>[2x]WELTILHTNDVHSRLEQTSEDSSKC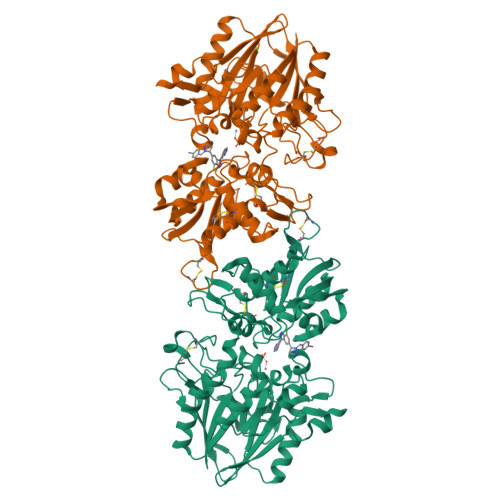VDASRCMGGVARLFTKVQQIRRAEPNVLLLDAGDQYQGTIWFTVYKGAEVAHFMNALRYDAMALGNHEFDNGVEGLIEPLLKEAKFPILSANIKAKGPLASQISGLYLPYKVLPVGDEVVGIVGYTSKETPFLSNPGTNLVFEDEITALQPEVDKLKTLNVNKIIALGHSGFEMDKLIAQKVRGVDVVVGGHSNTFLYTGNPPSKEVPAGKYPFIVTSDDGRKVPVVQAYAFGKYLGYLKIEFDERGNVISSHGNPILLDSSIPEDPSIKADINKWRIKLDDYSTQELGKTIVYLDGSSQSCRFRECNMGNLICDAMINNNLRHTDEMFWNHVSMCILNGGGIRSPIDERNDGTITWENLAAVLPFGGTFDLVQLKGSTLKKAFEHSVHRYGQSTGEFLQVGGIHVVYDLSRKPGDRVVKLDVLCTKCRVPSYDPLKMDEVYKVILPNFLANGGDGFQMIKDELLRHDSGDQDINVVSTYISKMKVIYPAVEGRIKFSGGGGAGGGGHHHHHH>GGSGPLKPEEHEDILNKLLDPELAQSERTEALQQLRVNYGSFVSEYNDLTKEAR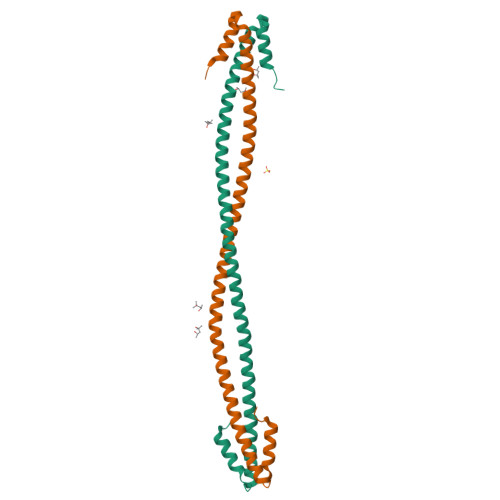SLSTELFKLKNAYEESLEHLETFKRENKNLQEEISDLTEQLGSSGKTIHELEKVRKQLEAEVEDLEKERDFYFGKLRNIELICQENEGENDPVLQRIVDILYATDEGFVIPD[4x]> SLSYSSQTSILPDAGDDFIVGDCLVYEDGVFEDPYLDKEVTQVAKQERKKNRRGGAKRLDESEIEPENLVPEEWRDIQAEVNLTKKDKRKIAQEMEFGVRVEKKRQGLIPLRKVDLNDFLTYKEAKLAQLRPVILDKPGNFSDDSGASSDGETAVSSPSERVAPKNPRWAVYGKGFDHVAKFFNSDKYDPSDKKSDGPRKLLSKEEKFMLNSRNPDLAVATSKKWLPLHTLAACGEFYLVDSLLKHNLDINATDVGGLTVLHRAIIGKKQAITNYLLRESANPFVLDDEGATLMHYAVQTASAPTIKLLLLYNADINAQDRDGWTPLHVAVQARRSDIVKLLLIKGADIEVKNKDGLTPLG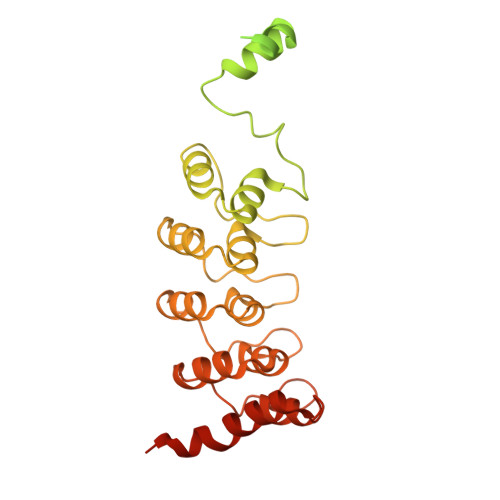LCLYLGREIRTYEVMKLLKEFPLSRHKKRLVTTDEDIE N-[1H-INDOL-3-YL-ACETYL]ASPARTIC 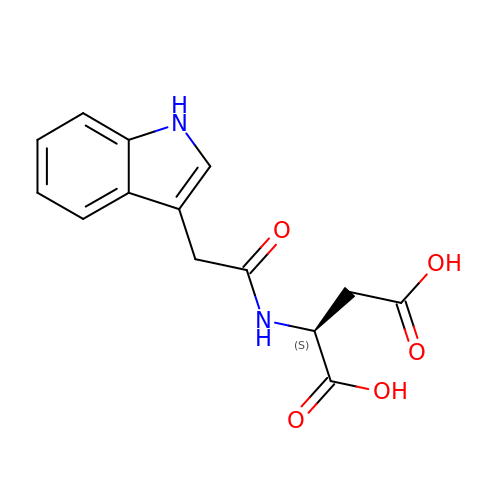ACID | C14 H14 N2 O5 | VAFNMNRKDDAKRM-NSHDSACASA-N2-AMINO-6-AMINOMETHYL-8-PHENYLSULFANYLMETHYL-3H-QUINAZOLIN-4-ONE 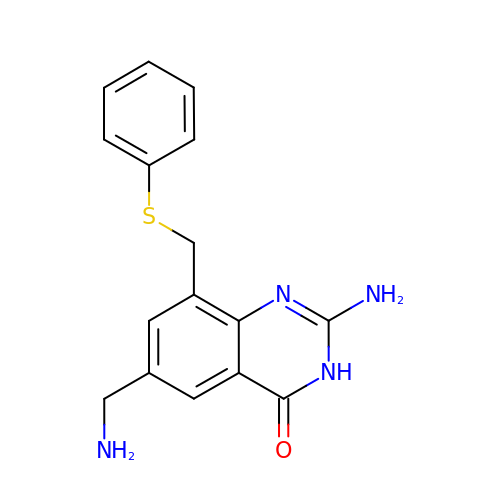| C16 H16 N4 O S | CBFXRTSHUMEYKQ-UHFFFAOYSA-N>[2x]MSEELVPHPNESLPGPRASPREVWKKGGRLLSVLLAVNVLLLACTLISGGAFNKVAVYDTDVFALLTTMMLLAALWIVFYLLRTARCPDAVPYRDAHAGP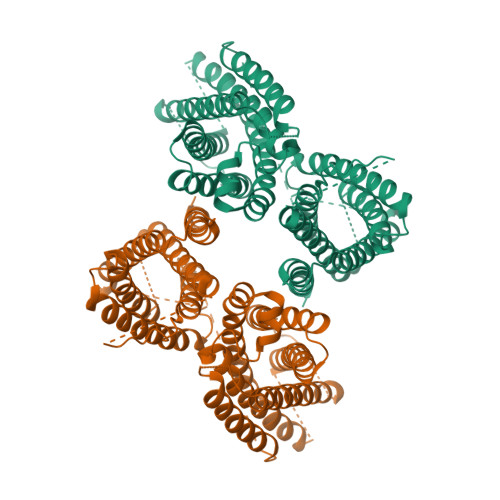IWLRGGLVLFGICTLVMDVFKTGYYSSFFECQSAIKILHPIIQAVFVIVQTYFLWISAKDCIHTHLDLTRCGLMFTLATNLAIWMAAVVDESVHQAHSYSGSHGNTSHTRLNPDSKRAGGAAEEDPCLCSTAICQIFQQGYFYLYPFNIEYSLFASTMLYVMWKNVGRLLASTHGHGHTPSRVSLFRETFFAGPVLGLLLFVVGLAVFILYEVQVSGERGHTRQALVIYYSFNIVCLGLMTLVSLSGSVIYRFDRRAMDHHKNPTRTLDVALLMGAALGQYAISYYSIVAVVVGSPRDLQGALNLSHALLMIAQHTFQNVFIIESLHRGPPGAEPREMPPKEPCQGITFANLDAIRTLPSCPPTPRLVIPNLESPQEAVAIISAPRCHWRRRCLKDISLFLLLCNVILWIMPAFGARPHFSNTVEVDFYGYSLWAAIVNICLPFGIFYRMHAVSSLLEVYVLS>[2x]NECLGTIGPVTPLDASDFALDIRMPGVTPKESD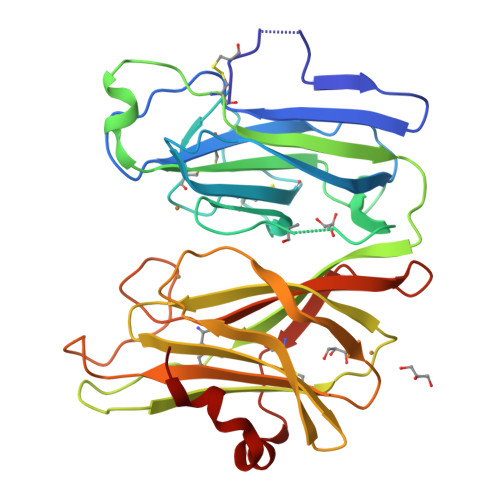TYFCMSMRLPVDEEAFVIDFKPRASMDTVHHMLLFGCNMPSSTGSYWFCDEGTCTDKANILYAWARNAPPTRLPKGVGFRVGGETGSKYFVLQVHYGDISAFRDNHKDCSGVSVHLTRVPQPLIAGMYLMMSVDTVIPPGEKVVNADISCQYKMYPMHVFAYRVHTHHLGKVVSGYRVRNGQWTLIGRQNPQLPAAFYPVEHPVDVTFGDILAARCVFTGEGRTEATHIGGTSSDEMCNLYIMYYMEAKYALSFMTCTKNVAPDMFRTIPAEANIPI> MANELTWHDVLAEEKQQPYFLNTLQTVASERQSGVTIYPPQKDVFNAFRFTELGDVKVVILGQDPYHGPGQAHGL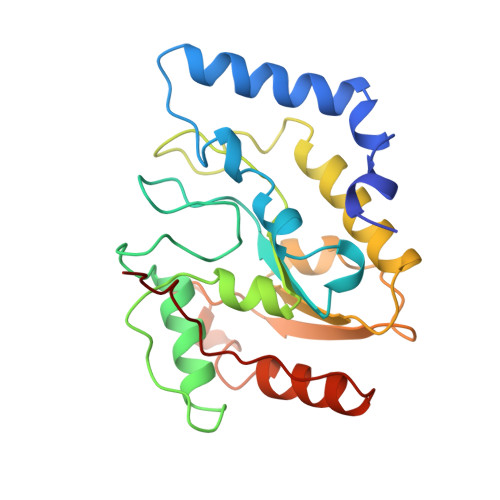AFSVRPGIAIPPSLLNMYKELENTIPGFTRPNHGYLESWARQGVLLLNTVLTVRAGQAHSHASLGWETFTDKVISLINQHREGVVFLLWGSHAQKKGAIIDKQRHHVLKAPHPSPLSAHRGFFGCNHFVLANQWLEQHGETPIDWMPVLPAESE>MSAQKRITLYMASASPFPHRVRLALEEAHATYEMIHISLVDKQDWYQKKVYPDRAQVPYLIYGGPELHPDEAPSPDAAKIPESLVILEFLADLFPAAHLLPSDPVLRARARLFTTAVETELLPAQKAFFLMGGPPDAMLAALDALQARLPPAGGFAAGPQWSIADAAVMPILLRLRMSVTLEVGFFAPGAAPVVRAALESPRFARLQRYIADNVARPSMAATWDEAAVKAEFVGRFEKLRSLKAAQHHHHHH[4x]

To further explore this issue, we have conducted biochemical and crystallographic studies on the interactions of six GSTOs from T. versicolor with chemical libraries. The six TvGSTOs (named TvGSTO1S to TvGSTO6S) used in this study are representatives of the twelve TvGSTOs that have a catalytic serine, while four others have a cysteine instead. In this study, we demonstrated at the biochemical and structural level that T. versicolor GSTs that belong to the Omega class interact with polyphenolic compounds found in wood, and in particular with flavonoids such as dihydrowogonin and naringenin. The ability of TvGSTOs to bind polyphenols through different sites suggests that fungal GSTs could be involved in the transport of various polyphenols.

In order to determine the structure of a complex between TvGSTO6S and a flavonoid, several candidate molecules were chosen for soaking experiments. Crystals of TvGSTO6S were unstable and brittle, and required some tricks to prepare complexes. Among the trials performed, one was successful where the droplet that gave rise to TvGSTO6S crystals was deposited for a few hours on a surface previously coated with naringenin (chemical structure in Supplementary Table S4). The structure of the complex was solved at a resolution of 2.3 Å. Two naringenin molecules bind in the pocket described above, which constitutes the L-site of TvGSTO6S. Each naringenin aromatic ring stacks with its symmetrical equivalent in an energetically-favored association (−13.64 kcal/mol calculated by DFT). In TvGSTO6S, the naringenin pair fits the apolar environment formed by the neighboring aliphatic part of the side chains of both monomers (L84, V85, R111, T115, E118 and T119) while a hydrogen bond with E88 stabilizes one of the flavonoid hydroxyl groups. For the first time in GSTs, one structure revealed a symmetrical ligandin site (L-site) filled with a pair of interacting ligands. In the case of TvGSTO6S, the L-site can host flavonoids.(3S,6S)-3-(4-hydroxybenzyl)-6-methylpiperazine-2,5-dione | 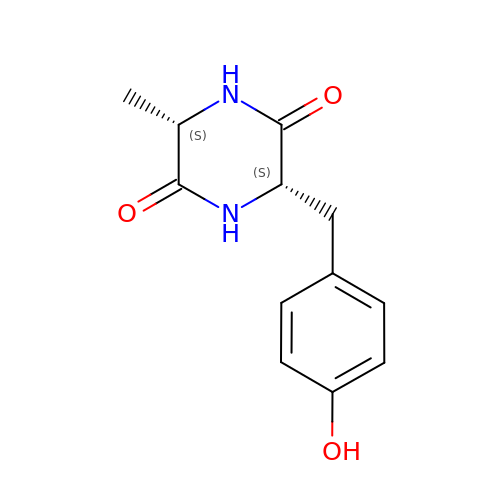C12 H14 N2 O3 | MFUNIDMQFPXVGU-XVKPBYJWSA-N> MLEQMISSSKVGVKINEWYKYIRLFSVPDSEILKAEVEEEIRHMKEDHDLLLYYSLMCFRHQLMLDYLEPKTLNEERPKISDLLEKIESSQTDLKGILEYYFNFFRGMYEFEQYEYLNAISFYKQAERKLSLVADEIERAEFHYKVAEIYYHMKQTHMSMHHIVQAIDSYKAHENYTVRVIQCSFVIGLNYLDMDYPEKAIPHFKNALDKAREIDMSRLIGSSLYNLGLCSFAEEAYEKASEYFKEGIRVYQDNGYEHSNRILDILLMLTKTTFKMRNHSEGISWCAHGLSLSKNLNDEIMAKMFEFIHALYVDNDNEKLNSILNYLELKSMLSDVEDL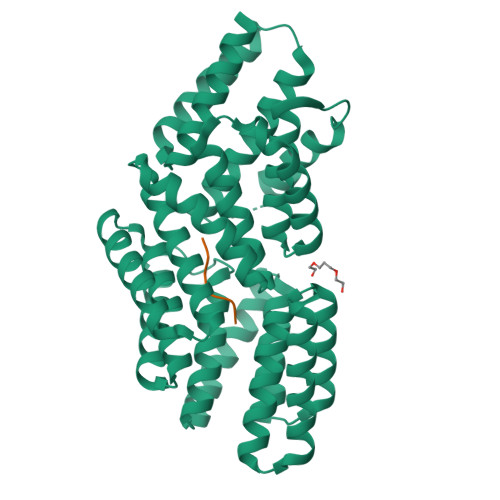ASDAAKYYNEKEDHKVAVAYYEKVLYARKQIQRGDCLYET;> RRGHTA> MAMYQQYSPKDVVCSWNGIAIEGFAPDSFLRLQRTSPLVTPVVGAGGQVALTRNADKTGTIEIELMQTSLSNQMLS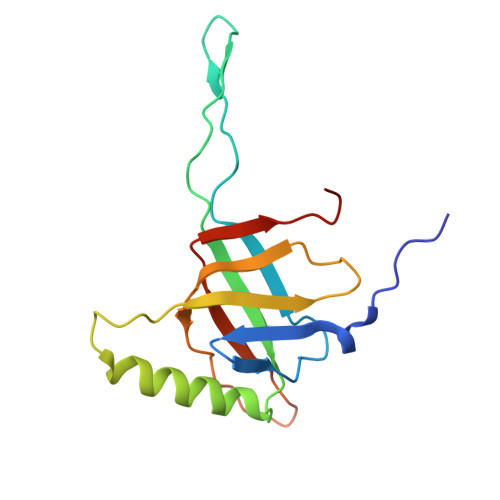AIQAKQDDMELEEDISSNFVIYDPSGSVLATGINAWLQELPQIELGRDQNSKTWIFGCEKLDYTSTIPASSV> MSSEKEELRERLVKICVENAKRKGDDTEEAREAAREAFELVREAAERAGIDSSEVLELAIRLIKECVENAQREGYDISEACRAAAEAFKRVAEAAKRAGITSSEVLELAIRLIKECVENAQRE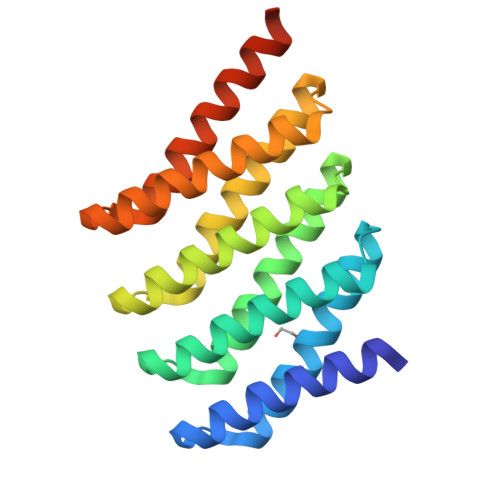GYDISEACRAAAEAFKRVAEAAKRAGITSSETLKRAIEEIRKRVEEAQREGNDISEACRQAAEEFRKKAEELKRRGDGWLEHHHHHH>MRLPRETDEEPEEPGRRGSFVEMVDNLRGKSGQGYYVEMTVGSPPQTLNILVDTGSSNFAVGAAPHPFLHRYYQRQLSSTYRDLRKGVYVPYTQGKWEGELGTDLVSIPHGPNVTVRANIAAITESDKFFINGSNWEGILGLAYAEIARPDDSLEPFFDSLVKQTHVPNLFSLQLCGAGFPLNQSEVLASVGGSMIIGGIDHSLYTGSLWYTPIRREWYYEVIIVRVEINGQDLKMDCKEYNYDKSIVDSGTTNLRLPKKVFE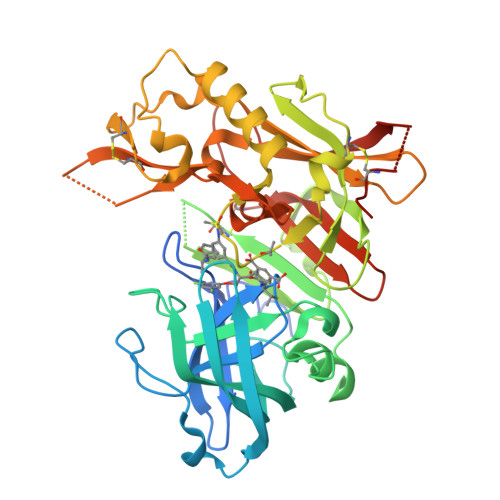AAVKSIKAASSTEKFPDGFWLGEQLVCWQAGTTPWNIFPVISLYLMGEVTNQSFRITILPQQYLRPVEDVATSQDDCYKFAISQSSTGTVMGAVIMEGFYVVFDRARKRIGFAVSACHVHDEFRTAAVEGPFVTLDMEDCGYN[3x]> GMELAEKDKGRDFTLRNARMDDIDQIIKINRLTLPENYPY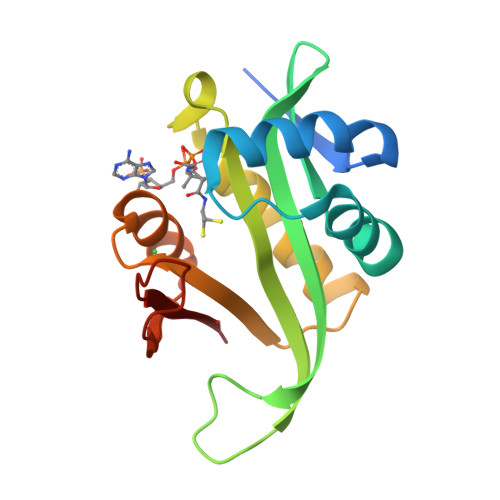YFFVEHLKEYGLAFFVAIVDNSVVGYIMPRIEWGFSNIKQLPSLVRKGHVVSIAVLEEYRRKGIATTLLEASMKSMKNDYNAEEIYLEVRVSNYPAIALYEKLNFKKVKVLKGYYADGEDAYLMARPL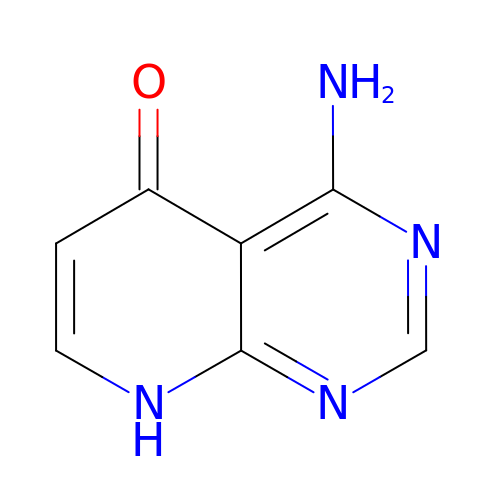4-aminopyrido[2,3-d]pyrimidin-5(8H)-one | C7 H6 N4 O | BGXMRRHONOWTLI-UHFFFAOYSA-N>MLSVLPLIDQAVAELAPGFRALSIVVQAAPLTQPEVARTALDRACQSVLAGGPAWGEAHLQQWADTFRQFGAKPQRTPCSAEALRKRVLRDGGLPSLDPVVDLYNAISIEYAIPVGGENIEAYVGSPRLVIADGSEPFDTMKEGAPAHEFPDAGEVVWRDDQGVTCRRWNWRQGVRTRLDADARHMWFILESLPAMPLEAL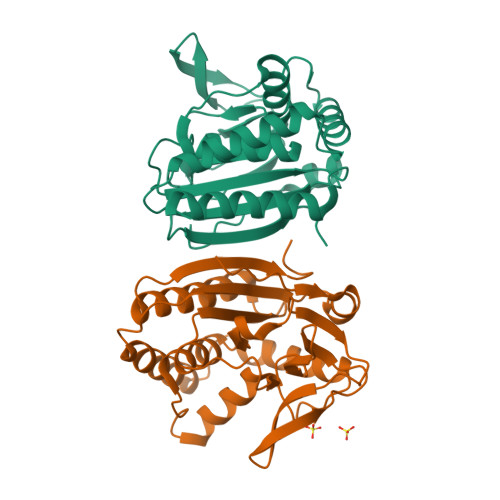TEAGDRLIEGLQAMMPGVQIESALVGPGGH[2x]> SSRKLTDISACSINIFYSTLGGSTQKFAEHVADRIRSSLQTELVEILNLDYIDLDEY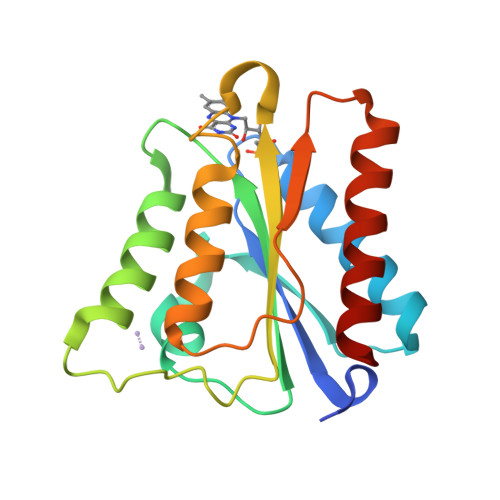FSKGNSNTVYLVLLPSYAIESSIDYFLSALQTTIDDFRIVARPLEKLRGFAVLGFGDFEQYAGDLFCYQAIAADQRLAKLGAQRIAPLGVVNVKLEKAQVYEAMEAWTDLFLQYAKEKA>[2x]MGS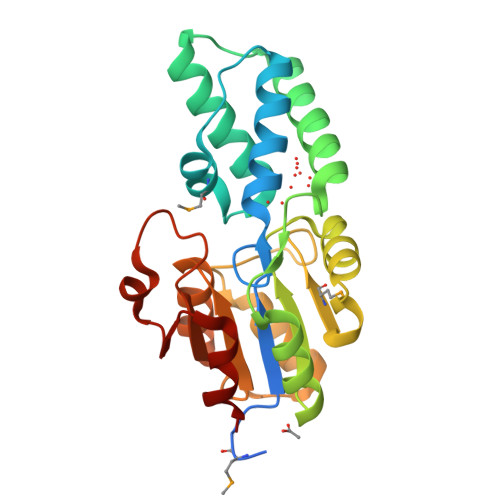DKIHHHHHHENLYFQGMTQFKLIGFDLDGTLVNSLPDLALSINSALKDVNLPQASENLVMTWIGNGADVLSQRAVDWACKQAEKELTEDEFKYFKRQFGFYYGENLCNISRLYPNVKETLEALKAQGYILAVVTNKPTKHVQPILTAFGIDHLFSEMLGGQSLPEIKPHPAPFYYLCGKFGLYPKQILFVGDSQNDIFAAHSAGCAVVGLTYGYNYNIPIAQSKPDWIFDDFADILKITQ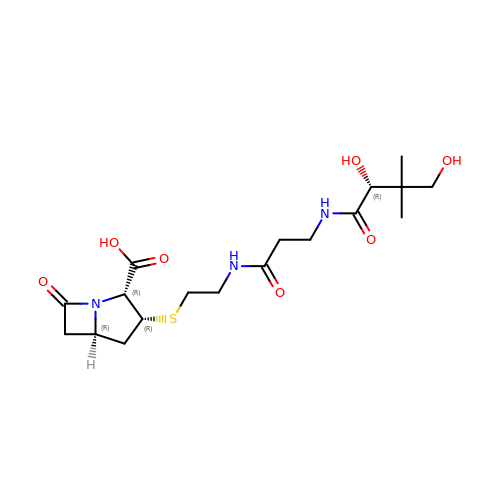(2R,3R,5R)-3-{[2-({N-[(2R)-2,4-dihydroxy-3,3-dimethylbutanoyl]-beta-alanyl}amino)ethyl]sulfanyl}-7-oxo-1-azabicyclo[3.2.0]heptane-2-carboxylic acid | C18 H29 N3 O7 S | XJMYKDFZQNYDFC-JLUCKKNBSA-N> AKWNPAGARRPVLDEAPVFYPTEEEFEDTLKYIESIRPMAEPYGICRIVPPSSWKPPCLLKDKSIWEGSKFSTRVQKVDKLQNRKSSKKGRRGGMMKRRKLAESEENSATAHTQTGMQQSPERFGFEPGPEFTLQTFQKYADDFSKQYFRKDTSMDSVPSVEDIEGEYWRIVEVPTEEIEVIYGADLETGTFGSGFPKLSPETKSDAEDKYAQSGWNLNNLPRLQGSVLSFEGGDISGVLVPWVYVGMCFSSFCWHVEDHHLYSLNYMHWGAPKLWYGVPGKDAVNLESAMRKHLPELFEEQPDLLHNLVTQFSPSLLKSEGVHVYRCVQHEGEFVLTFPRAYHAGFNCGFNCAEAVNVA

In this work we have identified a rice histone demethylase, namely JMJ703, which specifically demethylates methylated histone H3 lysine 4. Our results demonstrate that JMJ703 is essential for plant cell division and stem elongation and specifically demethylates mono-, di-, and trimethylated H3K4 in vivo and in vitro. Finally, the fragment spanning amino acids 139 to 498 (termed c-JMJ703), covering the JmjN and JmjC domains, was deemed to be suitable for crystallographic investigation. The c-JMJ703 molecule presented a canonical overall folding of JMJD2 proteins and contained four of the five domains defined in the structure of c-JMJD2A: the JmjN domain (A139-K199), the long β-hairpin (D200-T271), the mixed domain (L272-V377) and the JmjC domain (L378-A498).

The crystals belonged to the P63 space group with a slight change in unit cell parameters among the three crystals. The unambiguous electron density denoted Fe(II) (determined by inductively coupled plasma mass spectrometry) bound to c-JMJ703 and identified the active site within the JmjC domain. Three key residues, H394, E396, and H482, are perfectly conserved in JMJD2 proteins. They chelated Fe(II) in the active site through their hydrophilic side chains. Our data indicate that although most of the JMJ703 residues in α-KG/NOG stabilization showed a high structural similarity with JMJD2 proteins, the residues Y321 and N404 displayed specific features. Y321 and N404 showed significant conformational shifts compared with their counterparts in c-Rph1 and c-JMJD2A. The conformation of Y321 in c-JMJ703 indicates that the residue may not be in direct contact with α-KG or NOG.> RVLLALHDRAPQLKISDDRLTVVGEKGYSMVRASHGVRKGA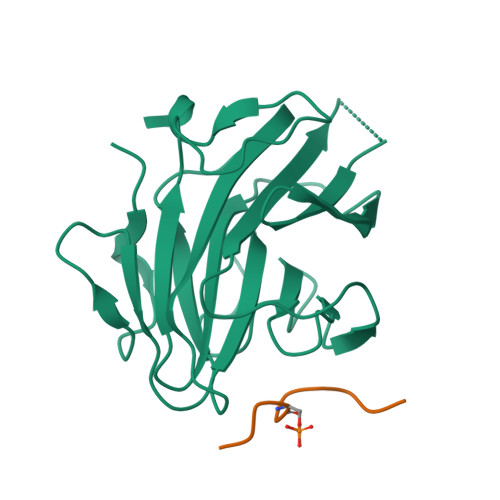WYFEITVDEMPPDTAARLGWSQPLGNLQAPLGYDKFSYSWRSKKGTKFHQSIGKHYSSGYGQGDVLGFYINLPEDISGRGSEIIFYKNGVNQGVAYKDIFEGVYFPAISLYKSCTVSINFGPCFKYPPKDLTYRPMSDMG;> ERESEFDIED>MFKMKVEDYFHDILRERKIHLTLIDPEEQTPEEAVEIARAAIRGGTDGIMLGGSTTDSSELDNTARALRENIDVPIILFPGNTTGVSRYADAIFFMSLLNSTNPYWIIGAQALGAATVKKMGIEALPMGYLVVEPGGTVGAVGDTKPVPRNKPDIAAAYAMAAEFLGMRLFYLEAGSGAPEHVPEEMIALVKRCTDQILIVGGGIRSGEDAARVAGAGADVVVTGTVVENSDNVEDKIREIVEGMGSV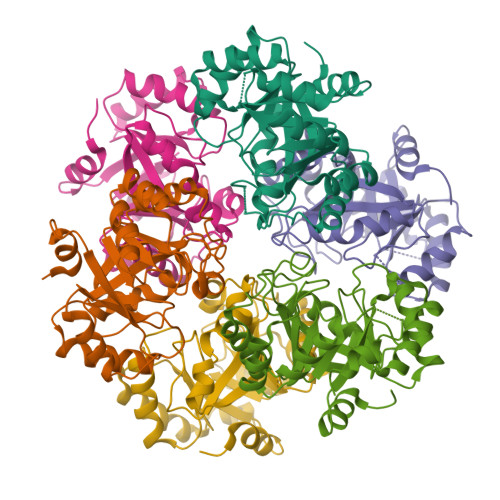LEHHHHHH[6x]>[3x]MAADAPAASQQSKPSESDKSESSMSSHAPVVFTLRTGIAEGRMVYIGVGGDIDRQVNPKLVVHEGETVQINLINGEGAQHDAVIDQYAARSAIV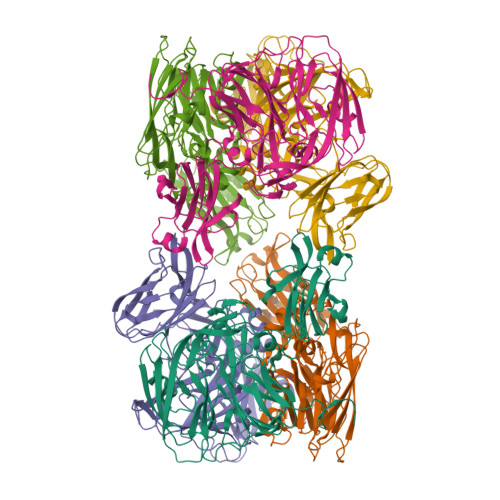SGKNASSTFSFIASKVGQFDYYCSLPGHRQAGMQGVLQVVPGNRAEMPSTAADITRDPADLPGPIGARQAKTVRIDLETVELKGQLDDKTTYTYWTFNGKVPGPFLRVRVGDTVELHLKNAKDSLMIHSVDFHGATGPGGAAAYTQTDPGAETVVTFKALVPGIFVYHCATPSVPNHITNGMYGLLLVEPEGGLPQVDREFYVMQGEIYTVKPFGTSGEQEMDYEKLISEKPEYFLFNGSVGALTRTHPLYANVGETVRIFFGVGGPNFTSSFHVIGEIFDHVYALGSVTSPPLTGVQTVSVPPGGATIVDFKLDRGGRYVLVDHALSRLDHGLVGFLNVDGPKNDAIMHEGPPKQENLYFQ> GSYDRNHTYIVSSLLEEPYLSLKQYTYGESLVGNDRFEGYCKDLADMLAAQLGIKYEIRLVQDGNYGAENQYAPGGWDGMVGELIRKEADIAISAMTITAERERVIDFSKPFMTLGISIMIKKGTPIKTPEDLTMQTDVNYGTLLYGSTWEFFRRSQIGLHNKMWEYMNANQHHSVHTYDEGIRRVRQSKGKYALLVE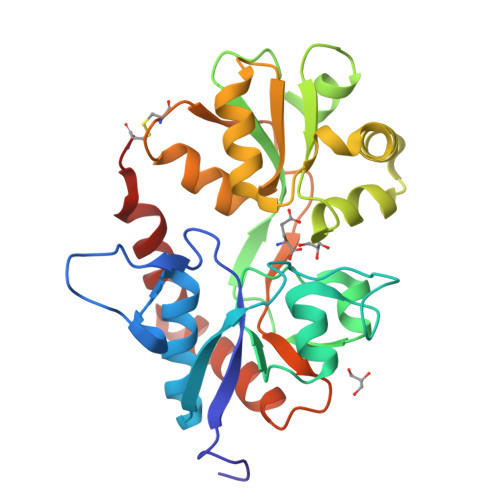SPKNEYVNARPPCDTMKVGRNIDTKGFGVATPIGSPLRKRLNEAVLTLKENGELLRIRNKWWFDKTECN> GPHMVKHPLNTAWTLWYTKPAVDKSESWSDLLRPVTSFQTVEEFWAII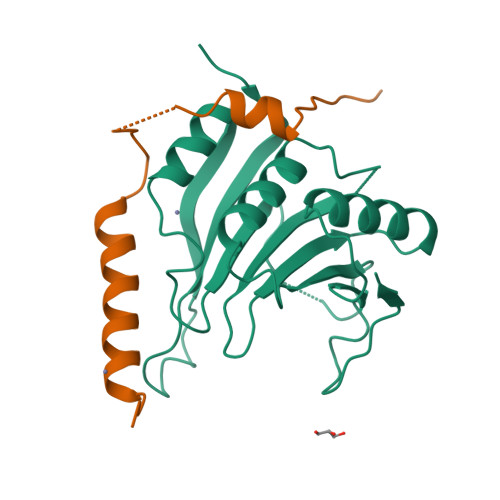QNIPEPHELPLKSDYHVFRNDVRPEWEDEANAKGGKWSFQLRGKGADIDELWLRTLLAVIGETIDEDDSQINGVVLSIRKGGNKFALWTASEDKEPLLRIGGKFKQVLALTDDGHLEFFPHSSANGRHPQPSITL;> GPHMIKYTIDELFQLKPSLTLEVNFDAVEFRAIIEKVKQLQHLKEEEFNSHH> MGAQVSSQKVGAHENTNVATGGSTVNYTTINYYKDSASNAASKLDFSQDPSKFTEPVKDIMIKTAP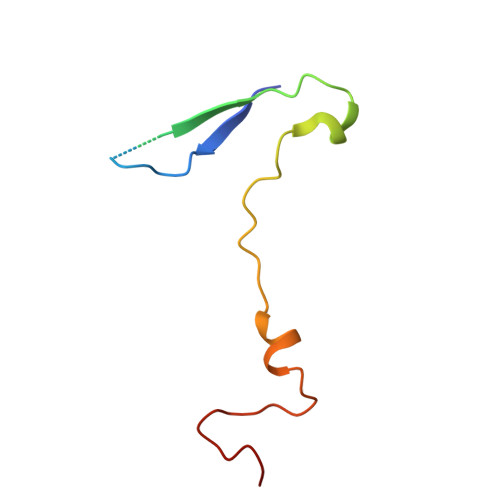ALN> VPLLRHDPLL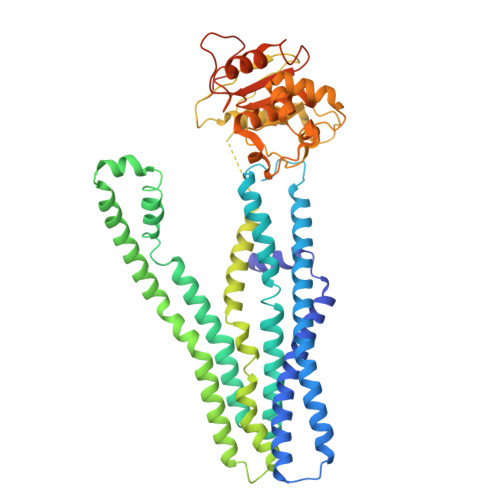RLTLELLRPRLGRFLLAAALGVLSLGSALALAGISAWLITRAWQMPPVLDLTVAVVAVRALGISRGVLGYCQRLASHDSALRAAANARTGLYRKLADAPPDEAMRLPSGELVARLGPAVDELADVLVRALLPIVVAVVLGCAAVGVIAVISPASAAVLAVCLVVAGVVAPALAARAAHASETVAAEHRSQRDTAGMLALEHAPELRVSGRLDSVIATFERHHRAWGEAADRAAAPAAVAAAMPTAAMGVSVVGAVIAGIALAPTVAPTTAAILMLLPLSAFEATTALPDAAAQLMRSRVAARRLLELTTPTPLRSRPDVATVDLAPGDRLAVVGPSGSGKTTMLMAIADRLNGAGGETPQRAAVFAEDAHLFDTTVRDNLLVVRGDATDTELVAALDRVGLGEWLAGLPDGLSTVLVGGAAAVSAGQRRRLLIARALISAFPVVLLDEPTENLDAGDARQMLEGLLTPGALFAADRTVVVATHHLPPGFDCPIVRCTGRLAVAGRYLGGIKAFDYKDDDDK> MSQGRLEERLTISKRELARLLKELKKWSAPATVLLSLYIPPGRPLSDVMTLLRQEYSITDNIKLKRTRQAVKRALSAAMDRLQMLTSTPPNGLVLFCGEDM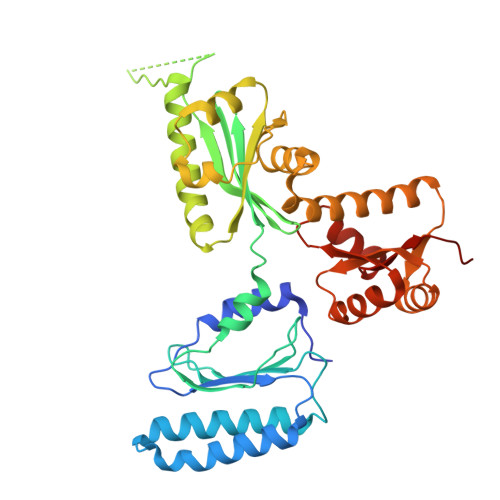STGKFECFMFSPPEPIRVFYYRTDKRFITDFLEDMVEDNNAIGIIIVERDQATIGLLKGARLEVLKELEGFVPGKHKMGGQSQRRYERIIEQMVDEFFKKVGEEASNLLVPLAEKGVLKGVIVAGPGLAKQEFVEGNYLDYRLKKILAPELVDVAYQGLQGLKEAVMKAEKVVEAQMYRDAVNAMEEFKLHLAKGTGMIVYGEKDVEAALEMGAVKTLLIHESREDLEEWVEKAKSSGAQVIVVPESLAEAEWFLKTFGGLAGILRFRISTV> MATYSLANERLRALEDIEREIGAILQNAGTAILELSKEKTNERLLDRQAAAFTTSVQHVEAELSAQIRYLTQVATGQPHEGSSYSSRKDCQMALKRVDYARLKI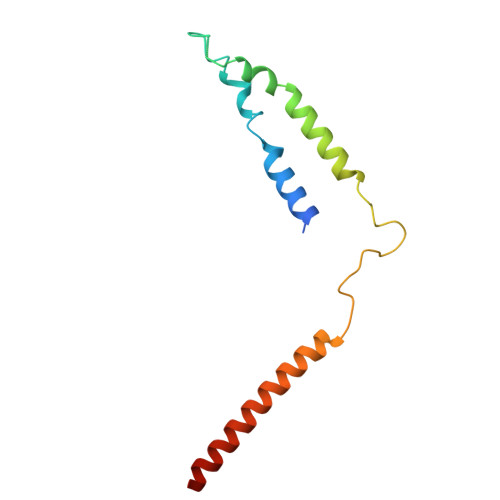SDVARTCEQMLEN> MVMGIFANCIFCLKVKYLPQQQKKKLQTDIKENGGKFSASLNPQCTHIILDNADVLSQYQLNSIQKNHVHIANPDFIWKSIREKRLLDVKNYDPYKPLDI

pmcPARP4 is an ADP-ribosyltransferase (ART) that uses NAD+ as substrate to add ADP-ribose onto target proteins, a process called mono(ADP-ribosylation) or MARylation. PARP4 is also referred to as vault PARP since it can localize to the vault particle, a cytoplasmic ribonucleoprotein complex. PARP4 has a distinct domain composition relative to other PARP enzymes; however, the N-terminal region of PARP4 is homologous to a collection of domains found in PARP1, a regulator of multiple nuclear processes including the cellular response to DNA damage. Collectively, the study establishes the human PARP4 BRCT as a nucleic acid–binding module.

However, the location of Phe39 on the potential nucleic acid–binding surface was intriguing so we also considered Phe39 as a possibly important residue. Conservation analysis using ConSurf indicated that Phe39 is conserved in 77% of 150 PARP4 homologs. We mutated Phe39 to glutamine and to alanine to test the importance of this region. We determined X-ray structures of the four PARP4 BRCT domain mutants. As expected from thermal stability analysis, the overall BRCT fold was not affected by the different mutations, and superposition of the mutant structures with WT BRCT yielded RMSD values between 0.5 and 0.8 Å (comparing all 763–788 atoms). Mutants F39A and F39Q both led to a shift in the position of the sidechain of K23, which impacted the charge distribution at the structure surface beyond just the F39 location. The loop that bears residue F39 was repositioned in the F39Q mutant, whereas this loop did not change in the F39A mutant, thus leading to visible changes in the electrostatic surface potential. Relative to WT BRCT (0.5 ± 0.2 μM), mutants F39Q and F39A exhibited slightly weakened binding, with estimated KD values of 0.9 ± 0.5 μM and 0.6 ± 0.1 μM, respectively. Relative to WT BRCT (KD of 19 ± 4 μM), F39Q and F39A showed weakened binding with KD values of 35 ± 10 μM and 33 ± 2 μM, respectively. The TM of WT BRCT was measured as 51.6 °C ± 0.2 deg, whereas TM values of 54.7 °C ± 0.4 deg, 54.3 °C ± 1 deg, 58 °C ± 1 deg, and 60.0 °C ± 0.7 deg were obtained for BRCT mutants F39A, F39Q, K31Q, and K23/24Q, respectively.>[2x]AFVQEPLPFDPGALEPYGMSAKTLEFHYGKHHKGYVDNLNKLTQDTELADKSLEDVIRTTYGDAAKVGIFNNAAQVWNHTFFWNSLKPGGGGVPTGDVAAR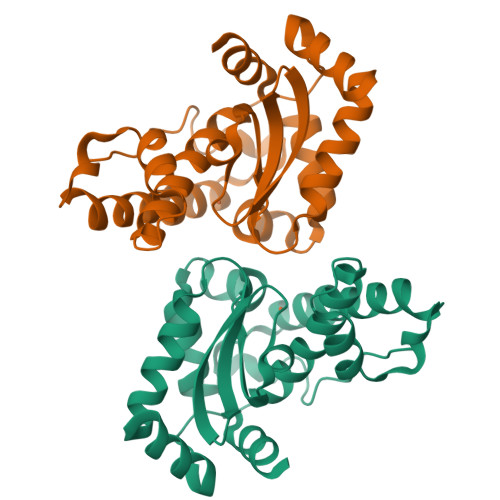INSAFGSYDEFKAQFKNAAATQFGSGWAWLVLEAGTLKVTKTANAENPLVHGQVPLLTIDVWEHAYYLDYQNRRPDFIDNFLNQLVNWDFVAKNLAAA> GSHMSNTQTVLPFTGLNTPSGVAVDSAGTVWVTDHGNNRVVKLAAGSNTQTVLPFTGLNTPSGVAVDSAGTVYVTDHGNNRVVKLAAGSNTQTVLPFTGLNTPSGVAVDSAGTVWVTDHGNNRVVKLAAGSNTQTVLPFTGLNTPSGV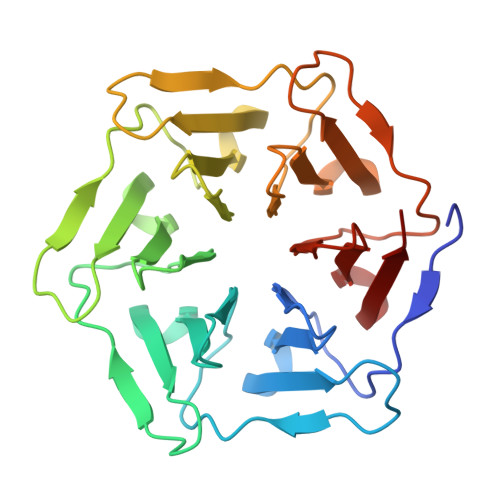AVDSAGTVYVTDHGNNRVVKLAAGSNTQTVLPFTGLNTPSGVAVDSAGTVWVTDHGNNRVVKLAAGSNTQTVLPFTGLNTPSGVAVDSAGTVYVTDHGNNRVVKLAAG> GPLGSEAHLYMQVQIVAEDQFCGHQGNDMYDEEKVKYTVFKVLKNSSLAEFVQSLSQTMGFPQDQIRLWPMQARSNGTKRPAMLDNEADGNKTMIELSDNENPWTIFLETVDPELAASGATLPKFDKDHDVMLFLKMYDPKTRSLNYCGHIYTPISCKIRDLLPVMCDRAGFIQDTSLILYEEVKPNLTERIQDYDVSLDKALDELMDGDIIVFQKDDPENDNSELPTAKEYFRDLYHRVDVIFCDKT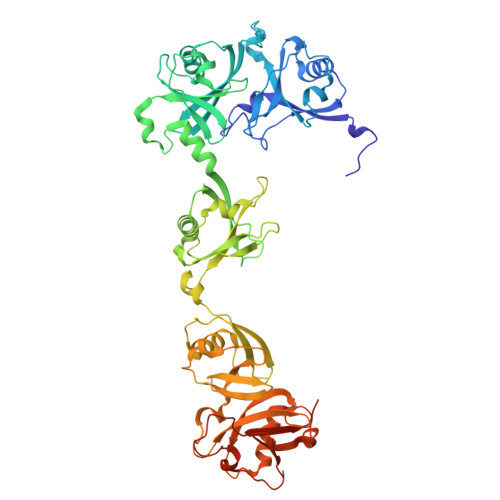IPNDPGFVVTLSNRMNYFQVAKTVAQRLNTDPMLLQFFKSQGYRDGPGNPLRHNYEGTLRDLLQFFKPRQPKKLYYQQLKMKITDFENRRSFKCIWLNSQFREEEITLYPDKHGCVRDLLEECKKAVELGEKASGKLRLLEIVSYKIIGVHQEDELLECLSPATSRTFRIEEIPLDQVDIDKENEMLVTVAHFHKEVFGTFGIPFLLRIHQGEHFREVMKRIQSLLDIQEKEFEKFKFAIVMMGRHQYINEDEYEVNLKDFEPQPGNMSHPRPWLGLDHFNKAPKRSRYTYLEKAIKIHN> HGSPVDICTAKPRDIPMNPMCIYRSPEKKATEDEGSEQKIPEATNRRVWELSKANSRFATTFYQHLADSKNDNDNIFLSPLSISTAFAMTKLGACNDTLQQLMEVFKFDTISEKTSDQIHFFFAKLNCRLYRKANKASKLVSANRLFGDKSLTFNETYQDISELVYGAKLQPLDFKENAEQSRAAINKWVSNKTEGRITDVIPSEAINVLV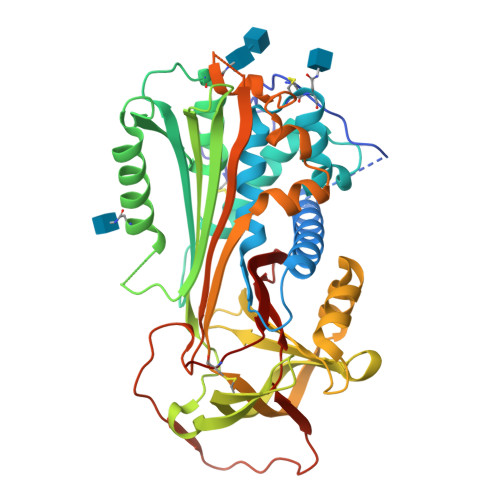LVNTRTSTVLVLVNTIYFKGLWKSKFSPENTRKELFYKADGESCSASMMYQEGKFRYRRVAEGTQVLELPFKGDDITMVLILPKPEKSLAKVEKELTPEVLQEWLDELEEMMLVVHMPRFRIEDGFSLKEQLQDMGLVDLFSPEKSKLPGIVAEGRDDLYVSDAFHKAFLEVNEEGSEAAASTAVVIAGRSLNPNRVTFKANRPFLVFIREVPLNTIIFMGRVANPCVK;> HGSPVDICTAKPRDIPMNPMCIYRSPEKKATEDEGSEQKIPEATNRRVWELSKANSRFATTFYQHLADSKNDNDNIFLSPLSISTAFAMTKLGACNDTLQQLMEVFKFDTISEKTSDQIHFFFAKLNCRLYRKANKSSKLVSANRLFGDKSLTFNETYQDISELVYGAKLQPLDFKENAEQSRAAINKWVSNKTEGRITDVIPSEAINELTVLVLVNTIYFKGLWKSKFSPENTRKELFYKADGESCSASMMYQEGKFRYRRVAEGTQVLELPFKGDDITMVLILPKPEKSLAKVEKELTPEVLQEWLDELEEMMLVVHMPRFRIEDGFSLKEQLQDMGLVDLFSPEKSKLPGIVAEGRDDLYVSDAFHKAFLEVNEEGSEAAASTAVVIAGRSLNPNRVTFKANRPFLVFIREVPLNTIIFMGRVANPCVK4-[3-(methylsulfonyl)phenoxy]-N-[(1S,3S,5S)-2-oxobicyclo[3.1.0]hexan-3-yl]butanamide | C17 H21 N O5 S | 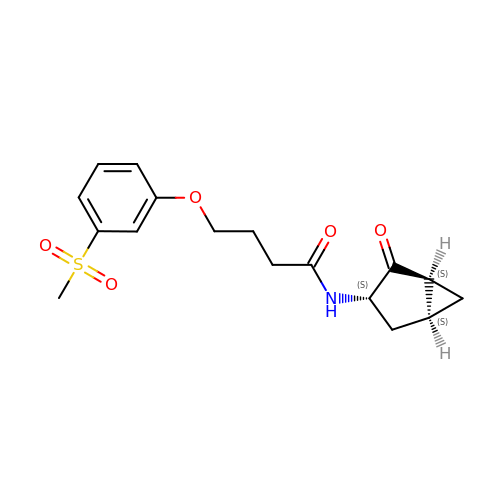MNLBJMNPVMBTLW-CQDKDKBSSA-N> SSDEEEARELIERAKEAAERAQEAAERTGDPRVRELARELKRLAQEAAEEVKRDPSSSDVNEALKLIVEAIEAAV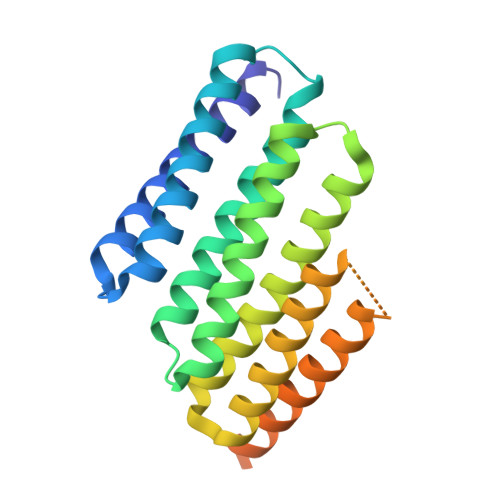DALEAAERTGDPEVRELARELVRLAVEAAEEVQRNPSSSDVNEALHSIVYAIEAAIFALEAAERTGDPEVRELARELVRLAVEAAEEVQRNPSSRNVEHALMRIVLAIYLAEENLREAEESGDPEKREKARERVREAVERAEEVQRDPSGWLNH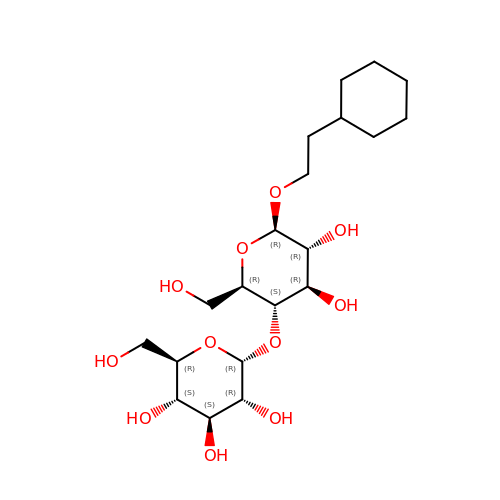2-(6-(2-CYCLOHEXYLETHOXY)-TETRAHYDRO-4,5-DIHYDROXY-2(HYDROXYMETHYL)-2H-PYRAN-3-YLOXY)-TETRAHYDRO-6(HYDROXYMETHYL)-2H-PYRAN-3,4,5-TRIOL | C20 H36 O11 | RHXPDNGQJSXOMW-OIIXUNCGSA-N> GGTISNNKAPIAKVTG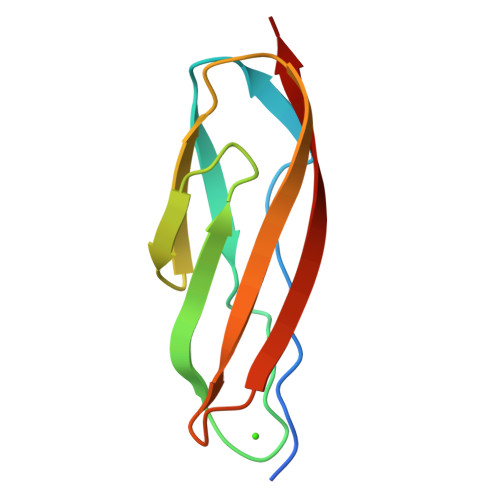PSTGAVGRNIEFSGKDSKDEDGKIVSYDWDFGDGATSRGKNSVHAYKKAGTYNVTLKVTDDKGATATESFTIEIKN>[2x]SLSSKDKDAVKALWGKIADKAEEIGADALGRMLAVYPQTKTYFSHWKDLSPGSAPV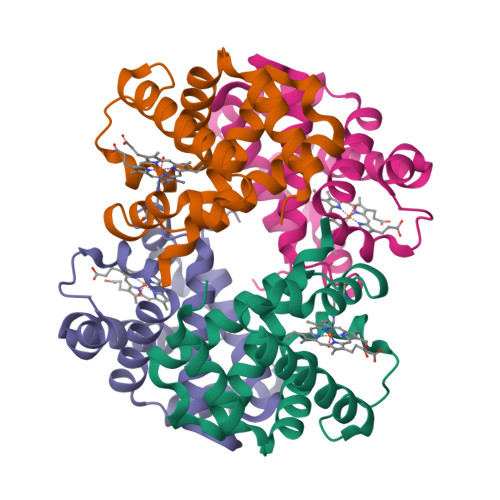NKHGKTIMGGLVDAVASIDDLNAGLLALSELHAFTLRVDPANFKILSHCILVQLAVKFPKDFTPEVHLSYDKFFSAVARALAEKYR;>VVWTDFERATIADIFSKLDYEAVGGATLARCLIVYPWTQRYFGNFGNLYNAAAIMGNPMIAKHGTTILHGLDRAVKNMDNIKATYAELSVLHSEKLHVDPDNFKLLSDCLTIVVAAQLGKAFSGEVQAAFQKFLSVVVSALGKQYH[2x]>M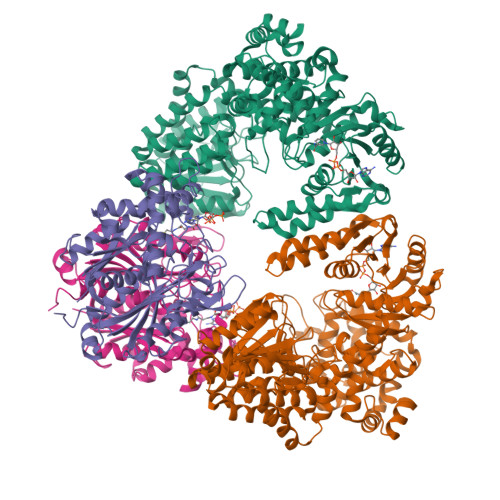IYEGKAITVTALESGIVELKFDLKGESVNKFNRLTLNELRQAVDAIKADASVKGVIVSSGKDVFIVGADITEFVENFKLPDAELIAGNLEANKIFSDFEDLNVPTVAAINGIALGGGLEMCLAADFRVMADSAKIGLPEVKLGIYPGFGGTVRLPRLIGVDNAVEWIASGKENRAEDALKVSAVDAVVTADKLGAAALDLIKRAISGELDYKAKRQPKLEKLKLNAIEQMMAFETAKGFVAGQAGPNYPAPVEAIKTIQKAANFGRDKALEVEAAGFAKLAKTSASNCLIGLFLNDQELKKKAKVYDKIAKDVKQAAVLGAGIMGGGIAYQSASKGTPILMKDINEHGIEQGLAEAAKLLVGRVDKGRMTPAKMAEVLNGIRPTLSYGDFGNVDLVVEAVVENPKVKQAVLAEVENHVREDAILASNTSTISISLLAKALKRPENFVGMHFFNPVHMMPLVEVIRGEKSSDLAVATTVAYAKKMGKNPIVVNDCPGFLVNRVLFPYFGGFAKLVSAGVDFVRIDKVMEKFGWPMGPAYLMDVVGIDTGHHGRDVMAEGFPDRMKDDRRSAIDALYEAKRLGQKNGKGFYAYEADKKGKQKKLVDSSVLEVLKPIVYEQRDVTDEDIINWMMIPLCLETVRCLEDGIVETAAEADMGLVYGIGFPLFRGGALRYIDSIGVAEFVALADQYAELGALYHPTAKLREMAKNGQSFFG[2x];>[2x]SLNPRDVVIVDFGRTPMGRSKGGMHRNTRAEDMSAHLISKVLERNSKVDPGEVEDVIWGCVNQTLEQGWNIARMASLMTQIPHTSAAQTVSRLCGSSMSALHTAAQAIMTGNGDVFVVGGVEHMGHVSMMHGVDPNPHMSLYAAKASGMMGLTAEMLGKMHGISREQQDAFAVRSHQLAHKATVEGKFKDEIIPMQGYDENGFLKIFDYDETIRPDTTLESLAALKPAFNPKGGTVTAGTSSQITDGASCMIVMSAQRAKDLGLEPLAVIRSMAVAGVDPAIMGYGPVPATQKALKRAGLNMADIDFIELNEAFAAQALPVLKDLKVLDKMNEKVNLHGGAIALGHPFGCSGARISGTLLNVMKQNGGTFGLSTMCIGLGQGIATVFERV>MLEQMISSSKVGVKINEWYKYIRLFSVPDSEILKAEVEEEIRHMKEDHDLLLYYSLMCFRHQLMLDYLEPKT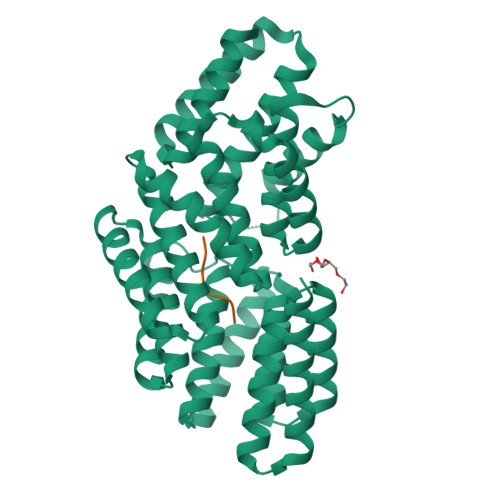LNEERPKISDLLEKIESSQTDLKGILEYYFNFFRGMYEFEQYEYLNAISFYKQAERKLSLVADEIERAEFHYKVAEIYYHMKQTHMSMHHIVQAIDSYKAHENYTVRVIQCSFVIGLNYLDMDYPEKAIPHFKNALDKAREIDMSRLIGSSLYNLGLCSFAEEAYEKASEYFKEGIRVYQDNGYEHSNRILDILLMLTKTTFKMRNHSEGISWCAHGLSLSKNLNDEIMAKMFEFIHALYVDNDNEKLNSILNYLELKSMLSDVEDLASDAAKYYNEKEDHKVAVAYYEKVLYARKQIQRGDCLYET[2x];>RRGHTAS[2x]>[7x]X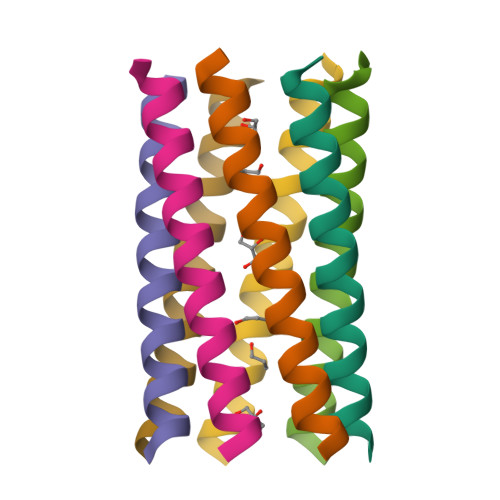GEIAQGIKEIAKGIKEIAWGIKEIAKGIKGX>[2x]APPSVFAEVPQAQPVLVFKLIADFREDPDPRKVNLGVGAYRTDDCQPWVLPVVRKVEQRIANNSSLNHEYLPILGLAEFRTCASRLALGDDSPALQEKRVGGVQSLGGTGALRIGAEFLARWYNGTNNKDTPVY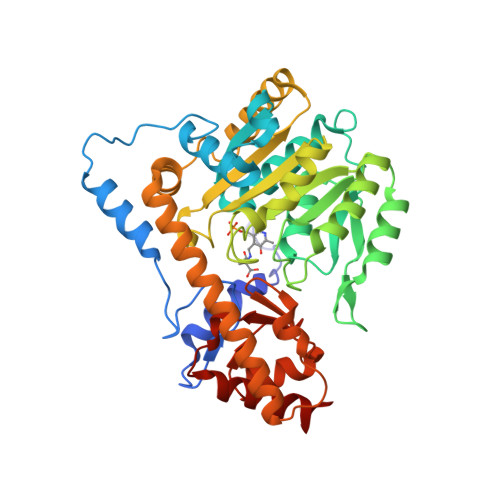VSSPTWENHNGVFTTAGFKDIRSYRYWDTEKRGLDLQGFLSDLENAPEFSIFVLHACAHNPTGTDPTPEQWKQIASVMKRRFLFPFFDSAYQGFASGNLEKDAWAIRYFVSEGFELFCAQSFSKNFGLYNERVGNLTVVAKEPDSILRVLSQMQKIVRVTWSNPPAQGARIVARTLSDPELFHEWTGNVKTMADRILSMRSELRARLEALKTPGTWNHITDQIGMFSFTGLNPKQVEYLINQKHIYLLPSGRINMCGLTTKNLDYVATSIHEAVTKIQ In Gram-positive bacteria, nitrogen homeostasis is controlled by an operon encoding glutamine synthetase (GS), a dodecameric machine that assimilates ammonium into glutamine, and the GlnR repressor. GlnR detects nitrogen excess indirectly by binding glutamine-feedback-inhibited-GS (FBI-GS), which activates its transcription-repression function. GS generates glutamine from glutamate, ATP, and ammonium by a mechanism that involves the initial phosphorylation of the γ-carboxyl group of glutamate by ATP and the subsequent incorporation of ammonium. The structures show FBI-GS binds the GlnR C-terminal domain within its active-site cavity, juxtaposing two GlnR monomers to form a DNA-binding-competent GlnR dimer.

To visualize the active, transition state (TS) conformations of the GS proteins we reacted them with l-methionine-S-sulfoximine (MSO) in the presence of ATP and solved the structures. In these structures, the Met-Sox-P methyl group occupies the ammonium substrate binding site, thus mimicking the GS transition state and preventing further reaction. Structures of the Pp, Lm, and Sa GS-Met-Sox-P-ADP complexes were obtained to 1.98, 3.50, and 2.95 Å resolution, respectively. Hence, the contacts in the Pp structure will be described here due to its higher resolution. In the complexes, the ADP adenine N6 is read by the carbonyl oxygen of Leu326. The side chains of Tyr199 and Arg329 make stacking interactions with the adenine base and Ser247 makes a hydrogen bond to the adenine N1 atom. Contacts to the Met-Sox-P phosphate are provided by Mg2+ ions and the side chains of GS residues Arg314, Arg329, Arg333, Arg334, and His243. The Arg296 side chain interacts with the Met-Sox carboxyl moiety and the Met-Sox-P amide nitrogen interacts with the Glu132 side chain as well as the carbonyl of Gly239. Catalytic E flap residue Glu302 contacts Asp52´ and is close to the Met-Sox-P methyl group. The Glu302–Asp52´ interaction would shield the Met-Sox-P from attack by bulk solvent as well as facilitate proton abstraction of the ammonium to form ammonia.

>MSYTREDIIRIAEEENVRFIRLQFTDLLGTIKNVEIPVSQLEKALDNKMMFDGSSIEGYVRIEESDMYLYPDLDTWVVFPWVTSDRVARLICDIYKPDGSPFAGDPRGILKRVLKEAEELGYTSMNVGPEPEFFLFKTDEKGDPTTELNDQGGYFDLAPMDLGENCRREIVLKLEEMGFEIEASHHEVAPGQHEIDFKYADAVKAADQIQTFKLVVKTIARQHGLHATFMPKPLFGVNGSGMHCNQSLFKDNENVFYDETDELGLSQTARHYMAGILKHARAMAAITNPTVNSYKRLVPGYEAPCYVAWSASNRSPMIRIPASRGLSTRVEVRNPDPAANPYLALAVMLRAGLDGIKRQMALPAPIDRNIYVMSEEERIEEGIPSLPADLKEALSELIRSEVISDALGDHALAYFYELKEIEWDMYRTQVHQWERDQYLTLY[3x]RtGH124 is the defining member of CAZY family GH124. Unusually for R. thermocellum, RtGH124A is not targeted to the multi-enzyme cellulosome complex of the organism but instead consists of a ‘dockerin’ domain which instead targets the enzyme to the cell surface of the bacterium, followed by a CAZY GH124 catalytic domain; RtGh124 is therefore an unusual enzyme if its primary role is in cellulose degradation yet it is not part of the cellulose complex. Here, we show that the metal-ion site of GH124 can accommodate a variety of metal ions (but not Ca2+) and that the histidine is modified by a carbonyl group at C2 to make 2-oxohistidine (but only at a fraction of approximately 0.5). Metal binding also occurs with a stoichiometry of approximately 0.5 (in solution by ITC and in the crystal through occupancy refinement) and we are thus unable to deconvolute whether the 2-oxohistidine is required for metal binding or antithetical to it.

Manganese is coordinated by Asp141, Gln172, Glu175, His176, His264 and a water molecule. In several structures with other metals, the water is at a very low occupancy or is absent, while Glu175 is often found in a double conformation, with only one of its positions coordinating the metal. The reasons for this are unclear: it may reflect pH, the partial metal occupancy or histidine modification. High-resolution structures of RtGH124 (1.40–0.94 Å) have revealed an unambiguous modification of C2 of His264. In the case of manganese, the metal and the His264 modification both display partial occupancies of 0.7 and 0.3, respectively. Occupancy values were similar for other metals under similar conditions, varying from 0 to 0.5 for the histidine modification and from 0 to 0.8 for the metal.

> GPAPANTQSGILNDGYFPPGTSKHELIARASSLKVSEVKAIIKKQVDEHWDVIRDVCGFKNKEVAYAFFFGMATRESTFRAATETGSGASHAFGPLQTAETAYANANPNYMPEHNVPEMHQYDFTEYNFYDVGISVHMGIRHFLHFARLAKEKYSGRDIARHGLMGYNTGWIDGADESWIVRYADETAALGAWYLRNNHMSDDEFTWDTDPRVDRSNPWEIYY>MGSIGIIIASHGEFAAGIHQSGSMIFGEQEKVQVVTFMPNEGPDDLYAKFNNAVAAFDAEDEVLVLADLWSGSPFNQASRVMGENPERKFAIITGLNLPMLIQAYTERLMDAAAGVEKVAANIIKEAKDGIKALP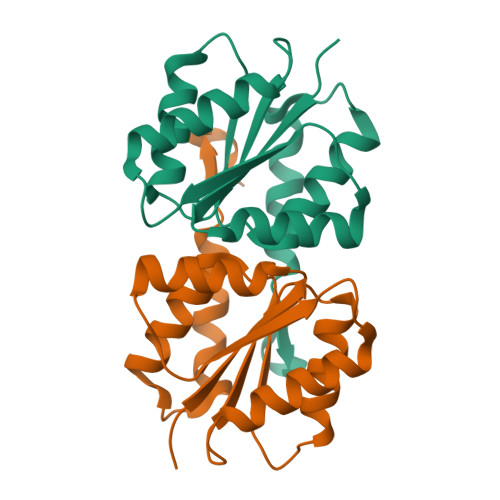EELNP[4x]[(3aR,4R,6R,6aR)-4-(6-aminopurin-9-yl)-2-oxidanyl-2-sulfanylidene-3a,4,6,6a-tetrahydrofuro[3,4-d][1,3,2]dioxaphosphol-6-yl]methanol | C10 H12 N5 O5 P S 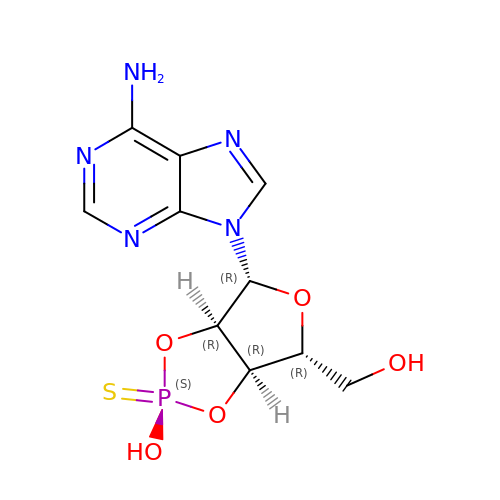| OMSUUENXGWGOLC-LHKKBNDGSA-N> NEAIKEDAGALSKAEPDDWEDAADIATPDLESANGDGVGTSMLDSGDRT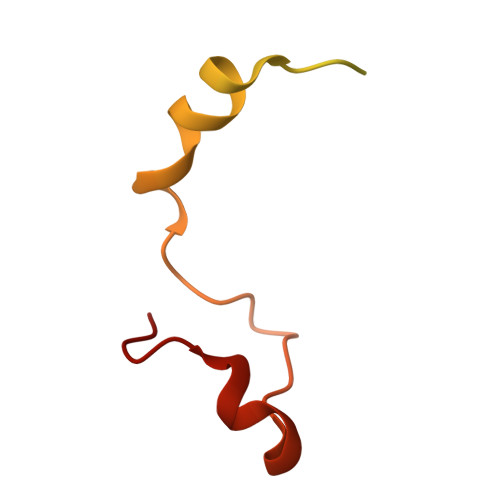GDMAKKYSRDFLLKFAEQFLDLPHNFEVTSDIESLMSTHTN AcrIIA15 is an anti-CRISPR (Acr) protein that inhibits Staphylococcus aureus Cas9 (SaCas9). The AcrIIA15 protein, consisting of 170 amino acids, is comprised of two domains: an N-terminal domain (NTD) from residues 1 to 56, which contains a HTH motif resembling a transcriptional repressor, and a C-terminal domain (CTD) from residues 57 to 170. AcrIIA15, by combining the HTH domain and Cas9 inhibitory domain within a single protein, exhibits dual functionality as a bi-functional anti-CRISPR protein capable of both transcriptional repression and CRISPR-based cleavage inhibition. Our structural and biochemical studies demonstrate that AcrIIA15 functions as a dimer to simultaneously inhibit both anti-CRISPR operon transcription and SaCas9-sgRNA DNA recognition.

To elucidate the molecular mechanisms underlying AcrIIA15 inhibition, we solved the cryo-EM structure of SaCas9-sgRNA-AcrIIA15CTD ternary complex at a resolution of 3.31 Å. In the ternary complex, one AcrIIA15CTD molecule binds to one SaCas9-sgRNA complex. AcrIIA15CTD is situated in the cleft between the PAM interacting (PI) and wedge (WED) domains of SaCas9. Notably, the PAM region of the target DNA would also be located within this same cleft between the PI and WED domains of SaCas9. AcrIIA15CTD is composed of five α-helices and a β-sheet consisting of three β-strands. The surface of AcrIIA15CTD carries a significant negative charge and resembles the size and shape of conventional B-form dsDNA. Specifically, the PAM recognition residues of SaCas9, N985 and N986, form hydrogen bonds with AcrIIA15 residues Y130 and D125, respectively, showing that AcrIIA15CTD binding directly blocks the PAM recognition sites in SaCas9. Specifically, the sidechain of D72 in AcrIIA15 forms hydrogen bonds with residue K50 of SaCas9, as well as with the base of G21, which is the first nucleotide of the repeat region in the sgRNA. Notably, mutations of AcrIIA15 residues Y161 and Y162, interacting with the sgRNA and the WED domain, completely abolished AcrIIA15CTD′s inhibitory activity. Taken together, our findings show that AcrIIA15CTD inhibits the DNA cleavage activity of SaCas9 by preventing it from binding to target DNA.

> MKRNYILGLDIGITSVGYGIIDYETRDVIDAGVRLFKEANVENNEGRRSKRGARRLKRRRRHRIQRVKKLLFDYNLLTDHSELSGINPYEARVKGLSQKLSEEEFSAALLHLAKRRGVHNVNEVEEDTGNELSTKEQISRNSKALEEKYVAELQLERLKKDGEVRGSINRFKTSDYVKEAKQLLKVQKAYHQLDQSFIDTYIDLLETRRTYYEGPGEGSPFGWKDIKEWYEMLMGHCTYFPEELRSVKYAYNADLYNALNDLNNLVITRDENEKLEYYEKFQIIENVFKQKKKPTLKQIAKEILVNEEDIKGYRVTSTGKPEFTNLKVYHDIKDITARKEIIENAELLDQIAKILTIYQSSEDIQEELTNLNSELTQEEIEQISNLKGYTGTHNLSLKAINLILDELWHTNDNQIAIFNRLKLVPKKVDLSQQKEIPTTLVDDFILSPVVKRSFIQSIKVINAIIKKYGLPNDIIIELAREKNSKDAQKMINEMQKRNRQTNERIEEIIRTTGKENAKYLIEKIKLHDMQEGKCLYSLEAIPLEDLLNNPFNYEVDHIIPRSVSFDNSFNNKVLVKQEENSKKGNRTPFQYLSSSDSKISYETFKKHILNLAKGKGRISKTKKEYLLEERDINRFSVQKDFINRNLVDTRYATRGLMNLLRSYFRVNNLDVKVKSINGGFTSFLRRKWKFKKERNKGYKHHAEDALIIANADFIFKEWKKLDKAKKVMENQMFEEKQAESMPEIETEQEYKEIFITPHQIKHIKDFKDYKYSHRVDKKPNRELINDTLYSTRKDDKGNTLIVNNLNGLYDKDNDKLKKLINKSPEKLLMYHHDPQTYQKLKLIMEQYGDEKNPLYKYYEETGNYLTKYSKKDNGPVIKKIKYYGNKLNAHLDITDDYPNSRNKVVKLSLKPYRFDVYLDNGVYKFVTVKNLDVIKKENYYEVNSKCYEEAKKLKKISNQAEFIASFYNNDLIKINGELYRVIGVNNDLLNRIEVNMIDITYREYLENMNDKRPPRIIKTIASKTQSIKKYSTDILGNLYEVKSKKHPQIIKKG;> MEKVDTWIVYRGRTADMNKSYIAEGSTYEEVYNNFVDKYGYDVLDEDIYEIQLLKKNGENLDDYDVDSDGINNYDKLDEFRESDYVDLEDYDYRELFENSSSQVYYHEFEITHE>MPKQTLDGNTAAAHVAYAMSEVATIYPITPSSPMAEIADEWAAHGRKNIFGKTLQVAEMQSEAGAAGAVHGSLAAGALTTTFTASQGLLLMIPNMYKIAGELLPCVFHVAARALSTHALSIFGDHADVMAARQTGFAMLSSASVQEVMDLAL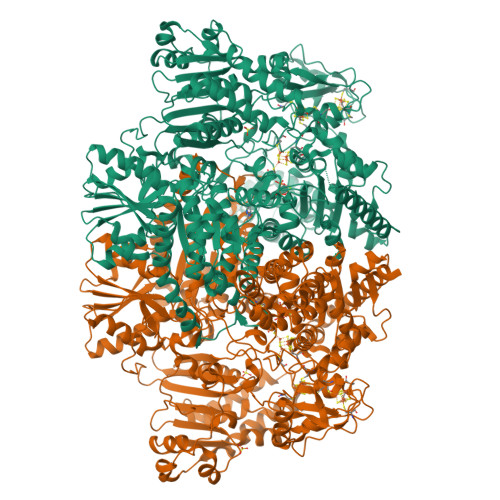VAHLATLKARVPFVHFFDGFRTSHEVQKIDVIEYEDMAKLVDWDAIRAFRQRALNPEHPHQRGTAQNPDIYFQSREAANPYYLATPGIVAQVMEQVAGLTGRHYHLFDYAGAPDAERVIVSMGSSCEVIEETVNYLVEKGEKVGLIKVRLFRPFSAEHFLKVLPASVKRIAVLDRTKEPGSLGEPLYEDVQTVLAEHGKNILVVGGRYGLGSKEFNPSMVKAVFDNLAATTPKNKFTVGITDDVTHTSLEIKEHIDTSPKGTFRCKFFGLGSDGTVGANKNSIKIIGDHTDMYAQGYFVYDSKKSGGVTISHLRFGKQPIQSAYLIDQADLIACHNPSYVGRYNLLEGIKPGGIFLLNSTWSAEEMDSRLPADMKRTIATKKLKFYNIDAVKIAQEIGLGSRINVIMQTAFFKIANVIPVDEAIKYIKDSIVKTYGKKGDKILNMNFAAVDRALEALEEIKYPASWADAVDEAAATVTEEPEFIQKVLRPINALKGDELPVSTFTPDGVFPVGTTKYEKRGIAVNIPQWQPENCIQCNQCSLVCPHAAIRPYLAKPADLAGAPETFVTKDAIGKEAAGLKFRIQVSPLDCTGCGNCADVCPAKVKALTMVPLEEVTAVEEANYNFAEQLPEVKVNFNPATVKGSQFRQPLLEFSGACAGCGETPYVKLVTQLFGDRMIIANATGCSSIWGGSAPACPYTVNRQGHGPAWASSLFEDNAEFGYGMALAVAKRQDELATAISKALEAPVSAAFKAACEGWLAGKDDADRSREYGDRIKALLPGEISQASGEVKDLLLDIDRQKDYLTKKSIWIIGGDGWAYDIGYGGLDHVLASGANVNVLVLDTEVYSNTGGQSSKATQTGAVARFAAGGKFTKKKDLGLMAMSYGYVYVASVAMGASHSQLMKALIEAEKYDGPSLIIAYAPCINHGINMTYSQREAKKAVEAGYWPLYRYNPQLAQEGKNPFILDYKTPTASFRDFLMGEIRYTSLKKQFPEKAEQLFAKAEADAKARLEQYKKLAEG[6x]>[2x]GSHMIKVLSPAKINLGLWVLGRLPSGYHEILTLYQEIPFYDEIYIREGVLRVETNIGIPQEENLVYKGL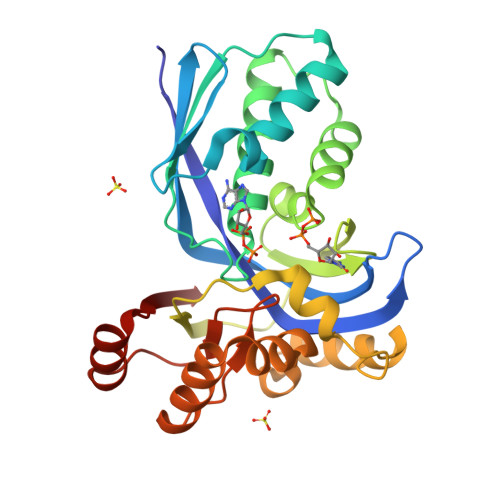REFERITGIEINYSIFIQKNIPPGAGLGGGSSNLAVVLKKVNELLGSPLSEEELRELVGSISADAPFFLLGKSAIGRGKGEVLEPVETEISGKITLVIPQVSSSTGRVYSSLREEHFVTPEYAEEKIQRIISGEVEEIENVLGDIARELYPEINEVYRFVEYLGFKPFVSGSGSTVYFFGGASEELKKAAKMRGWKVVELEL> MEDKNIVYGPEPFYPLEDGTAGEQLYKALKKYAQLPGTIALTDAHTEENIS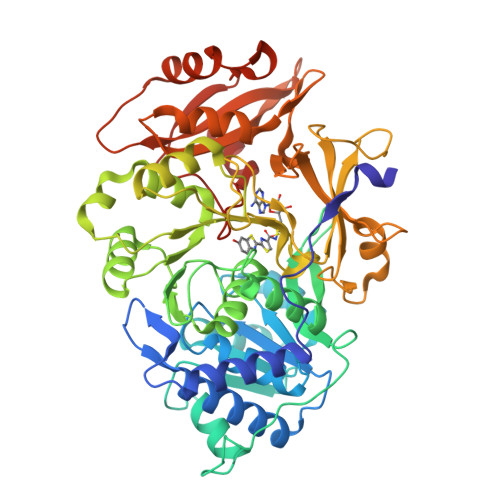YAELLELTCRLAESLKNYGLKQNNTIAVCSENNLQFFIPVIAALYIGVAVAPVNDKYTERELINSLNISKPTIIFCSKKTLQKILQVKKKLSYIKKIIILDSKEDIGGYQCLNNFISQHSDANFNVSNFKPNSFDRDEQVALIMNSSGTTGLPKGVMLTHKNLVVRFSHCRDPIFGNQIIPGTAILTVIPFHHGFGMFTTLGYFTCGFRIVLMHRFEEELFLKSLQDYKVQSTLLVPTLMAFFAKSPLVDKYDLSNLKEIASGGAPLSKEVGEAVAKRFKLPGIRQGYGLTETTSAIIITPEGDVKPGSTGKVVPFFSAKVVDLDTGKTLGPNQRGELCFKGDMIMKGYVNNPEATKEIIDKDGWLHSGDIGYYDEDGHFFIVDRLKSLIKYKGYQVAPAELESILLQHPSIIDAGVTGIPDEDAGELPAACVVLQPGKHLTEKEVIDYVASQVSSAKRLRGGVRFVDEIPKGSTGKIDRKALRQILQKQKSKL> CGC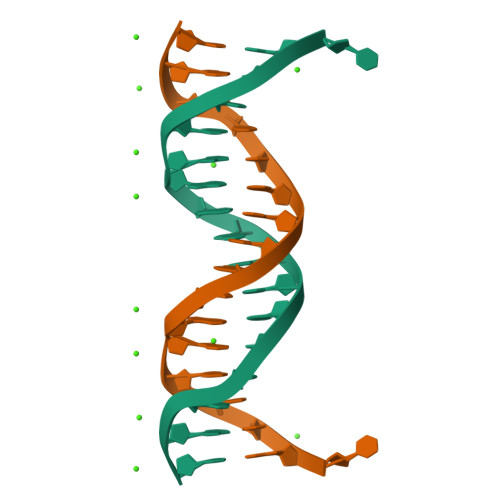TGGAAATTTCCAGC BbvCI, a Type IIT restriction endonuclease, recognizes and cleaves the seven base pair sequence 5′-CCTCAGC-3′, generating 3-base, 5′-overhangs. BbvCI is composed of two protein subunits, each containing one catalytic site. Either site can be inactivated by mutation resulting in enzyme variants that nick DNA in a strand-specific manner. Earlier mutagenesis of these residues confirmed their catalytic nature and demonstrated that the site in the R1 subunit cleaves the bottom strand of the target site, while the site in the R2 subunit cleaves the top strand.

Subsequently, crystals of the BbvCI enzyme were grown at near-neutral pH. The crystals corresponded to space group P32, with four subunits (i.e. a single enzymatic tetramer) in the asymmetric unit. The crystals diffracted to only 3.8 Å resolution; nevertheless, they produced an obvious molecular replacement solution using the previously determined structure of the R2 homodimer as a search model. In the resulting maps, electron density corresponding to two additional protein chains was clearly present, and this was used to build models of two additional R1 subunits. In the resulting hetero-tetramer, the two R2 subunits occupy the same positions and orientations as they do in the R2 homodimer. The pronounced concave surface present between the two R2 subunits is also present between the two R1 subunits. These surfaces pack against one another at a ∼45° angle in the tetramer, forming an X-shaped dimer of dimers. In the hetero-tetramer, two deep grooves are present on opposite sides of the molecule, each formed by residues from one R1 subunit, and one R2 subunit. Within each groove, the catalytic site residues of one subunit are exposed on one side, and those of the other subunit are exposed diagonally across on the other side. These paired sites occur ∼25 Å apart in opposing orientations, appropriately positioned to cleave double stranded DNA to produce a 3-base, 5′-overhang. Out of the entire calculated buried interfacial surface area and corresponding free energy of association for the tetramer (5094 Å2; –37 kcal/mol), a substantial contribution is made by the R2–R2 interface (1838 Å2; –32 kcal/mol), whereas all other interfaces in the tetramer contribute ∼600–900 Å2 that are predicted to add a few extra kcal/mol of association energy.

>MINEDFFIYEQLSHKKNLEQKGKNAFDEETEELVRQAKSGYHAFIEGINYDEVTKLDLNSSVAALEDYISIAKEIEKKHKMFNWRSDYAGSIIPEFLYRIVHVATVKAGLKPIFSTRNTIIEISGAAHREGLQIRRKNEDFALGFHEVDVKIASESHRVISLAVACEVKTNIDKNKLNGLDFSAERMKRTYPGSAYFLITETLDFSPDENHSSGLIDEIYVLRKQVRTKNRVQKAPLCPSVFAELLEDILEISYRASNVKGHVYDRLEGGKLIRV[2x];>[2x]MFNQFNPLVYTHGGKLERKSKKDKTASKVFEEFGVMEAYNCWKEASLCIQQRDKDSVLKLVAALNTYKDAVEPIFDSRLNSAQEVLQPSILEEFFEYLFSRIDSIVGVNIPIRHPAKGYLSLSFNPHNIETLIQSPEYTVRAKDHDFIIGGSAKLTIQGHGGEGETTNIVVPAVAIECKRYLERNMLDECAGTAERLKRATPYCLYFVVAEYLKLDDGAPELTEIDEIYILRHQRNSERNKPGFKPNPIDGELIWDLYQEVMNHLGKIWWDPNSALQRGKVFNRP>[2x]GNLREVRYHDEERPYFIDWDFALRKSGANQTESSMHMQSVVPSSPATPVENDFKRIHSISDMTYLARRTRDEPIRKGVIVPCKDLLDAEEALSRALEVLPLAHKETKDKDRKQQPGIAADLAQRRRPGTPLRLEGIGELSAVVNVAVRDAEGKNDEEILALIKPWVQNSKADLLARRVRRLTFICGRNDGSYPSYYTFRGPDYAEDDSIRHIEPSLAFQLELGRLSKFKLTPVFTQNKNIHVYEAVGRGVETDRRYFTRAVVRPGRLRDEISTAEYLISEADRVVNDIFDALEIIGTNKTDLNHMFINFSHTFQVTADEVAESLQGFLDRFGPRGWRLRVHQVEIRINCMRSDNNDENDTMPLRVIITNTSGFVIQIELYEEKLSEKGEWVYYYVSGNAKIGSMHLLPVSTPYPTKNWLQPKRYKAHILGTQYVYDFPELFRQAIQNSWTEAVKKIPSLAAKQPAIGECIDYNELVLGDQDNLAEVSREPGMNSTGMVGWLINARTPEYPDGRKFIVVANDITFKIGSFGPKEDTFFFKCTELARKM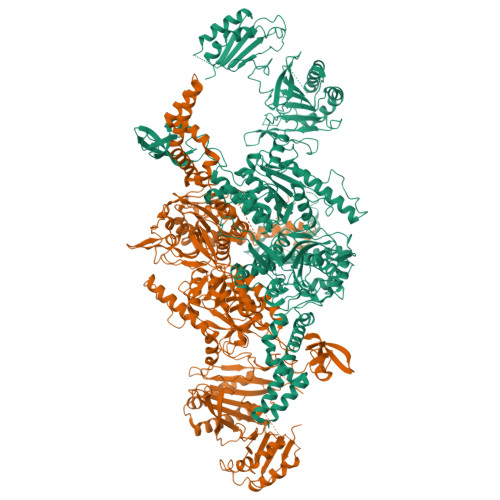GIPRIYLSANSGARLGLAEELMPHFNVAWNDPAKPEAGFKYLYLSDEAKRRFENEVITEEIVEDGEKRHKIITIVGAEEGLGVECLRGSGLIAGATSRAYNDIFTCTLVTCRSVGIGAYLVRLGQRAVQVEGQPIILTGAPALNSLLGREVYTSNLQLGGTQIMYRNGVSHLTAKDDFDGVTKIVQWLSFIPDQRNNPLPILSPSPDPWDRDVVYTPPYKQTYDVRWMIAGKEDEDGFQPGLFDKDSFVETLGGWARTVVVGRARLGGIPMGVIAVETRTIENITPADPANPDSIEQVTNEAGGVWYPNSAFKTAQAINDFNYGEQLPLMILANWRGFSGGQRDMYNEVLKYGSFIVDALTRFEKPIFIYIPPHGELRGGSWVVVDPTINPASMEMYADEEARGGVLEPEGIIPIKYKKDKQLETMARLDPVYRSLKKEMAKEGLSKEESDNIKKKMQQREELLLPIYHQICVQFADLHDRAGRMKAKGVIRQSLQWRQSRRFFYWRVRRRLIEDDILRRIEEAINPAGKRRHDPENTSLAASPETRSPHLVQLESWVGIPGFKTNDREVVEWYEQNQDRINEKLEKLKKESIADQMRELLRAAEXXXXXXXXXXXXXXXXXXXXXXXXXXX>[4x]GSSHHHHHHSSGLVPRGSHMKSTSVSPFHLPLNH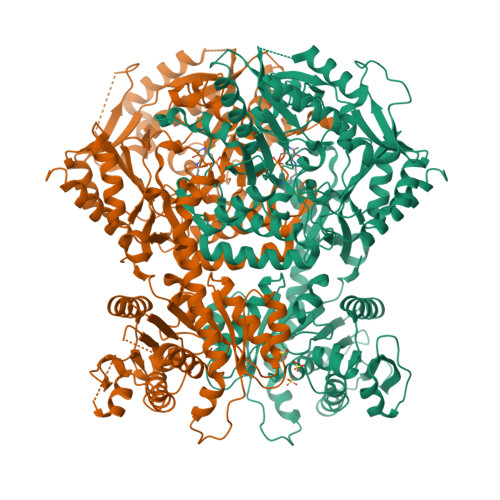PTYLIWSANTSLGKTLVSTGIAASFLLQQPSSSATKLLYLKPIQTGFPSDSDSRFVFSKLDSLSLRRQIPISISNSVLHSSLPAAKSLGLNVEVSESGMCSLNFRDEKTVTGAPELLCKTLYAWEAAISPHLAAERENATVEDSVVLQMIEKCLKEEMECGVKSEKSDLLCLVETAGGVASPGPSGTLQCDLYRPFRLPGILVGDGRLGGISGTIAAYESLKLRGYDIAAVVFEDHGLVNEVPLTSYLRNKVPVLVLPPVPKDPSDDLIEWFVESDGVFKALKETMVLANLERLERLNGMAKLAGEVFWWPFTQHKLVHQETVTVIDSRCGENFSIYKASDNSSLSQQFDACASWWTQGPDPTFQAELAREMGYTAARFGHVMFPENVYEPALKCAELLLDGVGKGWASRVYFSDNGSTAIEIALKMAFRKFCVDHNFCEATEEEKHIVVKVIALRGSYHGDTLGAMEAQAPSPYTGFLQQPWYTGRGLFLDPPTVFLSNGSWNISLPESFSEIAPEYGTFTSRDEIFDKSRDASTLARIYSAYLSKHLQEHSGVRQSAHVGALIIEPVIHGAGGMHMVDPLFQRVLVNECRNRKIPVIFDEVFTGFWRLGVETTTELLGCKPDIACFAKLLTGGMVPLAVTLATDAVFDSFSGDSKLKALLHGHSYSAHAMGCATAAKAIQWFKDPETNHNITSQGKTLRELWDEELVQQISSHSAVQRVVVIGTLFALELKADASNSGYASLYAKSLLIMLREDGIFTRPLGNVIYLMCGPCTSPEICRRLLTKLYKRLGEFNRT Recently, we characterized TgCyp23 among the various Cyps of the parasite, demonstrating its high PPIase activity and its ability to bind cyclosporin A (CsA), a well‐known inhibitor of Cyps (Favretto et al., 2023). TgCyp23 exhibits the typical eight‐stranded antiparallel β‐barrel structure, with two α‐helices flanking the barrel on either side, all of them connected by loops. TgCyp23 shows remarkable sequence identity with human CypA (~52% of identity) but has a 40‐aminoacid N‐terminal extension. Here, three new structures of the protein in complex with the three non‐immunosuppressive derivatives NIM811, dhCsA, and Alisporivir have been solved at 1.17, 1.20, and 1.20 Å resolution, respectively.

NIM811, a CsA derivative where N‐methylleucine (MeLeu‐4) is replaced by N‐methylisoleucine (MeIle‐4) at position 4, retains full capacity to inhibit CypA PPIase activity with a Ki value of 2.1 nM but possesses significantly reduced immunosuppressive activity (Schiene‐Fischer et al., 2022; Ptak et al., 2008). The MeLeu‐4 residue of CsA is replaced by MeIle‐4 in NIM811. This amino acid has a bulkier side chain that could provoke clashes with the Trp352 residue of the cavity. Superimposition of the TgCyp23:Alisporivir and TgCyp23:NIM811 complexes onto the structure of the CypA–CsA–CN ternary complex (Huai et al., 2002) clearly reveals that the side chain of MeIle‐4 in NIM811 and NEV‐4 in Alisporivir cannot enter the Cn hydrophobic cavity to establish a proper interaction. We observed a steric clash with the Trp352 aromatic ring that constitutes one wall of the Cn pocket. The MeIle‐4 side chain of NIM811 and NEV‐4 side chain of Alisporivir prevent the TgCyp23–drug complex from interacting with Cn. Remarkably, both NIM811 and dhCsA closely resembled the TgCyp23:CsA complex, implying that chemical modifications at position 4 of CsA exert negligible influence on the binding to the protein. NIM811, dhCsA, and Alisporivir are attached to the CsA binding pocket. Remarkably, all the modifications in the non‐immunosuppressive derivatives are exposed, protrude from the binding site, and are not involved in the crystal packing. All three compounds inhibit the catalytic activity of TgCyp23, with IC50 values between 0.8 and 2 nM, with Alisporivir having the highest inhibitory activity.

>GHMAPAPPANSGESSLLSESELPAGISYAEAMEGGSRPLLHPDNPVVFFDISIGSHEAGRIKIELFKNLAPKSAENFRQFCTGEFRQNQVPIGYKGATFHRIIKNFMIQGGDFVKGDGTGRLSIYGSSFPDEAFVLPHFRSGLLSLANSGPDTNGCQFFITCAKCDWLNRKHVVFGQVLGKESMQVVRKIEHVTVDGGNRPRIPVTVTQCGEL[2x];>[2x]ALLVTAGIVLA> MPALTKSQTDRLEVLLNPKDEISLNSGKPFRELESELLSRRKKDLQQIYAEERENYLGKLEREITRFFVDRGFLEIKSPILIPLEYIERMGIDNDTELSKQIFRVDKNFCLRPMLAPNLYNYLRKLDRALPDPIKIFEIGPCYRKESDGKEHLEEFTMLAFAQMGSGCTRENLESIITDFLNHLG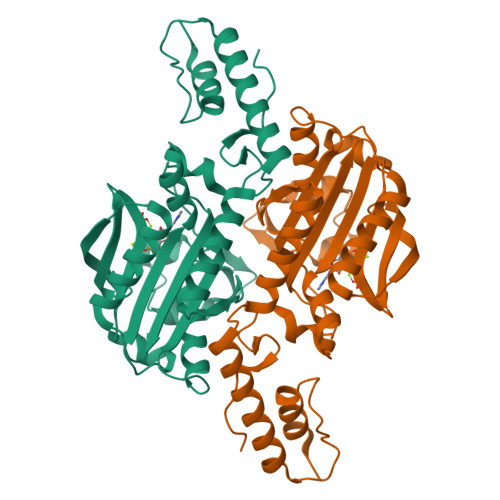IDFKIVGDSCMVYGDTLDVMHGDLELSSAVVGPIPLDREWGIDKPWIGAGFGLERLLKVKHDFKNIKRAARSESYYNGISTNLHHHHHH> DIEKYVEELYKVVKKIYEKTGTPIKFWDLVPD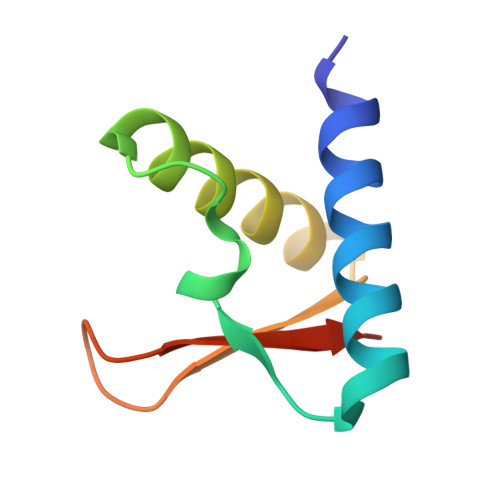VEPKIIARTFLYLLFLENMGRVEIIQEEPFGEILVVPMVDKL> MTVRKNQATLTADEKRRFVAAVLELKRSGRYDEFVRTHNEFIMSDTDSGERTGHRSPSFLPWHRRFLLDFEQALQSVDSSVTLPYWDWSADRTVRASLWAPDFLGGTGRSTDGRVMDGPFAASTGNWPINVRVDSRTYLRRSLGGSVAELPTRAEVESVLAISAYDLPPYNSASEGFRNHLEGWRGVNLHNRVHVWVGGQMATGVSPNDPVFWLHHAYVDKLWAEWQRRHPDSAYVPTGGTPDVVDLNETM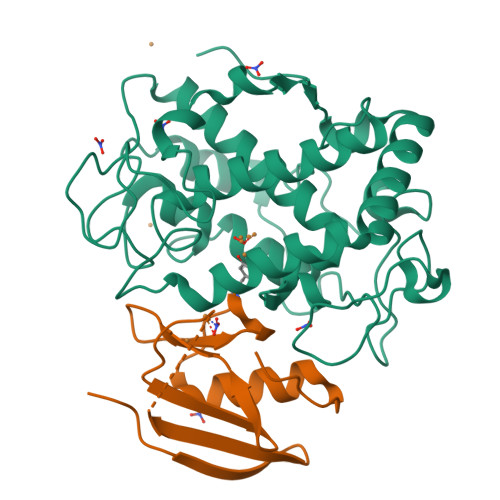KPWNTVRPADLLDHTAYYTFDALEHHHHHH;> MPEITRRRALTAAAAVAATASAAVTLAAPAASAAGHHEPAAPESFDEVYKGRRIQGRPARGAAHHHEHGGGYEVFVDGVQLHVMRNADGSWISVVSHYDPVPTPRAAARAAVDELQGAPLLPFPANLEHHHHHH The major regulator of virulence factors in L. monocytogenes is the transcription activator PrfA, a member of the Crp/Fnr family of regulators. PrfAWT is a homodimer in which each monomer consists of an N-terminal domain (residues 1 to 108) and a C-terminal DNA-binding domain (residues 138 to 237) linked by a long α-helix (αC, residues 109 to 137). Two α-helices in the C-terminal domain, αE (residues 170 to 178) and αF (residues 183 to 197), constitute the two helices of the typical HTH motif present in many prokaryotic transcription factors. Glutathione binding stabilizes the DNA-binding helix-turn-helix (HTH) motif in a conformation compatible with DNA-binding, thereby allowing expression of PrfA-regulated virulence factors.

The prfA gene modifications included three previously characterized amino acid substitutions as follows: four of the ten mutants carried the Gly to Ser substitution at residue 145 (PrfAG145S), one carried the Gly to Cys substitution at residue 145 (PrfAG145C), and two carried the Leu to Phe substitution at residue 140 (PrfAL140F). All the previously identified PrfA* mutants, i.e., PrfAG145S, PrfAG145C, and PrfAL140F, could grow in this medium with G-6-P, as could the PrfA mutants PrfAL140H and PrfAA218G, whereas the strain carrying the PrfAA94V mutation was unable to grow. The PrfAG145S, PrfAG145C, and PrfAL140F mutants showed the highest expression levels, followed by PrfAA218G and PrfAL140H. When grown in BHI supplemented with Amberlite XAD4 (BHIA), the wild-type and PrfAL140F mutant strains showed significantly increased expression of ActA compared to bacteria grown in only the BHI. To gain a deeper understanding of the PrfA* mutant proteins, the crystal structures of purified PrfAL140H, PrfAL140F, and PrfAA218G were determined as individual proteins and in complex with the PrfA hly promoter DNA. We expected that the crystal structures of PrfAL140H, PrfAL140F, and PrfAA218G would be similar to the PrfAG145S structure, since our in vivo characterization classified them as PrfA* mutations. However, their structures showed that each of the PrfA* variants had only one folded HTH motif, with the remaining structure residing in the PrfAWT conformation. The PrfAL140H, PrfAL140F, and PrfAA218G PrfA* mutants all had a folded HTH motif in one monomer of the homodimer but an uncollapsed central core structure. Consequently, we suggest that these mutant structures represent an intermediately activated form of the protein with features characteristic of both inactive and activated PrfA. When superimposed on monomer B, the recognition helix in monomer A is shifted up to 6 Å.

>GAMNAQAEEFKKYLETNGIKPKQFHKKELIFNQWDPQEYCIFLYDGITKLTSISENGTIMNLQYYKGAFVIMSGFIDTETSVGYYNLEVISEQATAYVIKINELKELLSKNLTHFFYVFQTLQKQVSYSLAKFNDFSINGKFGSICGQLLILTYVYGKETPDGIKITLDNLTMQELGYSSGIAHSSAVSRIISKLKQEKVIVYKNSCFYVQNLDYLKRYAPKLDEWFYLACPATWGKLN[2x]1-(2,5-dideoxy-5-pyrrolidin-1-yl-beta-L-erythro-pentofuranosyl)-5-methylpyrimidine-2,4(1H,3H)-dione | C14 H21 N3 O4 | 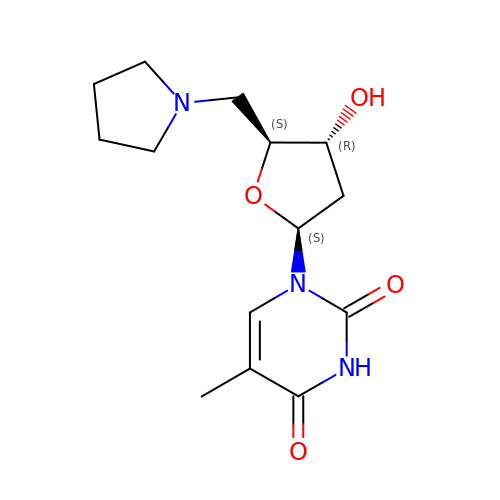XUSBTLVYPZUOAW-WOPDTQHZSA-N>SSPVAQKYDYILVGGGTAACVLANRLSADGSKRVLVLEAGPDNTSRDVKIPAAITRLFRSPLDWNLFSELQEQLAERQIYMARGRLLGGSSATNAT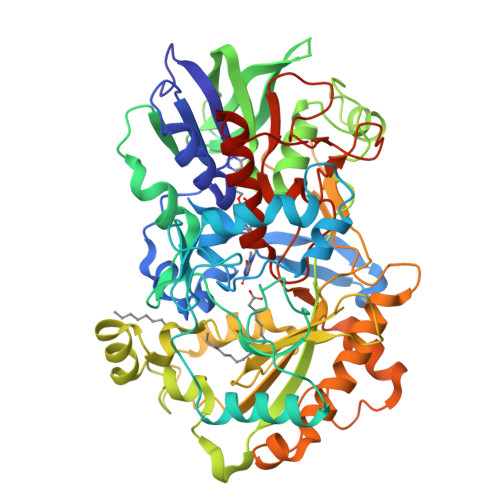LYHRGAAGDYDAWGVEGWSSEDVLSWFVQAETNADFGPGAYHGSGGPMRVENPRYTNKQLHTAFFKAAEEVGLTPNSDFNDWSHDHAGYGTFQVMQDKGTRADMYRQYLKPVLGRRNLQVLTGAAVTKVNIDQAAGKAQALGVEFSTDGPTGERLSAELAPGGEVIMCAGAVHTPFLLKHSGVGPSAELKEFGIPVVSNLAGVGQNLQDQPACLTAAPVKEKYDGIAISDHIYNEKGQIRKRAIASYLLGGRGGLTSTGCDRGAFVRTAGQALPDLQVRFVPGMALDPDGVSTYVRFAKFQSQGLKWPSGITMQLIACRPQSTGSVGLKSADPFAPPKLSPGYLTDKDGADLATLRKGIHWARDVARSSALSEYLDGELFPGSGVVSDDQIDEYIRRSIHSSNAITGTCKMGNAGDSSSVVDNQLRVHGVEGLRVVDASVVPKIPGGQTGAPVVMIAERAAALLTGKATIGASAAAPATVAA[2x]> SCKAFQGQTLREHIEAMLAAWEIVKNKYIPSIIRVMKTVGVKFTEEDADKFMKTLIILHDVGKCSEVYQKHLSNNEPLRGFRHELVSAYYAYNILKDMFKDETIAFIGALVVMMHHEPILMGQIRSLDKEELTPEVVLDKLRTFNGVMEGTESFIKSMIKEKLGVIPKVPSPTQEDVLREVIRLSVLARHRPDSGKLRMVVGALLI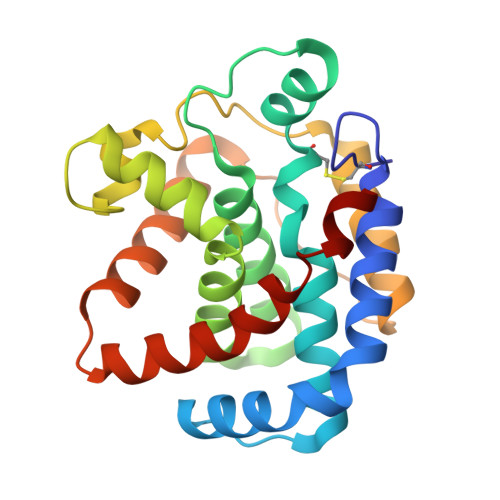PLVCDYKGAAAAA> MSQFTLYKNKDKSSAKTYPYFVDVQSDLLDNLNTRLVIPLTPIELLDKKAPSHLCPTIHIDEGDFIMLTQQMT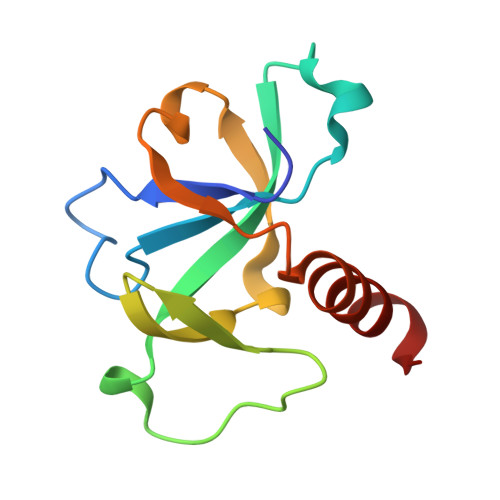SVPVKILSEPVNELSTFRNEIIAAIDFLITGI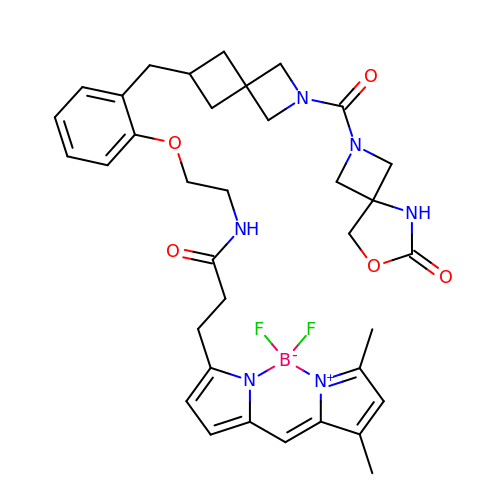3-[2,2-bis(fluoranyl)-10,12-dimethyl-1$l^{4},3-diaza-2$l^{4}-boratricyclo[7.3.0.0^{3,7}]dodeca-1(12),4,6,8,10-pentaen-4-yl]-~{N}-[2-[2-[[2-[(6-oxidanylidene-7-oxa-2,5-diazaspiro[3.4]octan-2-yl)carbonyl]-2-azaspiro[3.3]heptan-6-yl]methyl]phenoxy]ethyl]propanamide | C35 H41 B F2 N6 O5 | IREDGWRMCRGHGX-UHFFFAOYSA-N> VANTTYKAPIERPEDFLKDKEKAKEWERKEAERIEQKLERSEKEALESYKKDSVEISKYSQTRNYFYDYQIEANSREKEYKELRNAISKNKIDKPMYVYYFESPEKFAFNKVIRTENQNEISLEKFNEFKETIQNKLFKQDGFKDISLYEPGKGDEKPTPLLMHLKLPRNTGMLPYTNTNNVSTLIEQGYSIKIDKIVRIVIDGKHYIKAEASVVSSLDFKDDVSKGDSWGKANYNDWSNKLTPNELADVNDYM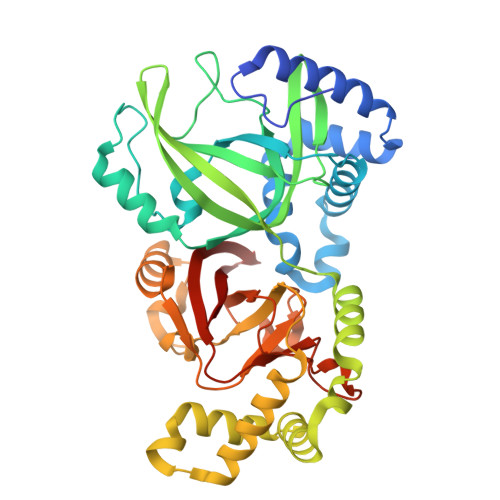RGGYTAINNYLISNGPVNNPNPELDSKITNIENALKREPIPTNLTVYRRSGPQEFGLTLTSPEYDFNKLENIDAFKSKWEGQALSYPNFISTSIGSVNMSAFAKRKIVLRITIPKGSPGAYLSAIPGYAGEYEVLLNHGSKFKINKIDSYKDGTITKLIVDATLIP> GAMDPEFLDPQLPPSSNFDLSAWYLSVPTDNNGDGKADSIKENDLNAGYADGTYFYTAADGGMVFRCPIDGYKTSTNTSYTRTELREMLRRGDTSIATQGVNGNNWVFGSAPASAREAAGGVDGVLRATLAVNHVTTTGDSG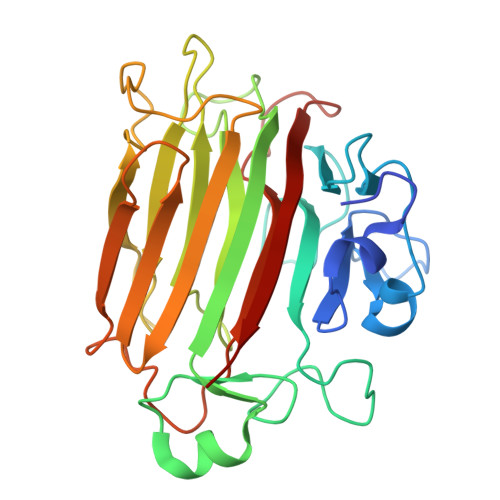QVGRVIVGQIHANNDEPLRLYYRKLPGHSKGSVYIAHEPNGGSDSWYDMIGSRSSSASDPSDGIALDEVWSYEVKVVGNTLTVTIFRAGKDDVVQVVDMGNSGYDVADQYQYFKAGVYNQNNTGNASDYVQVTFYALEQSHD>[2x]GMTRQRIAIDMDEVLADTLGAVVKAVNERADLNIKMESLNGKKLKHMIPEHEGLVMDILKEPGFFRNLDVMPHAQEVVKQLNEHYDI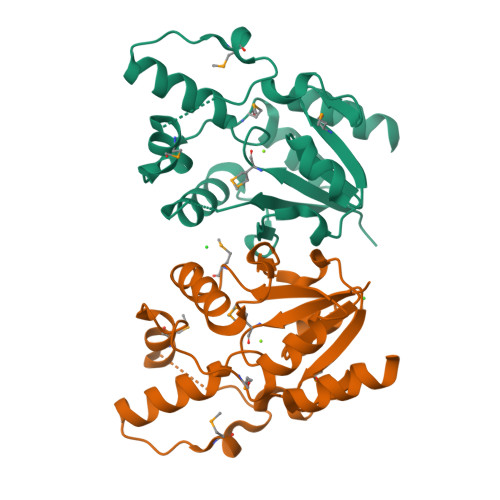YIATAAMDVPTSFHDKYEWLLEYFPFLDPQHFVFCGRKNIILADYLIDDNPKQLEIFEGKSIMFTASHNVYEHRFERVSGWRDVKNYFNSIEK>HAALRQPQVAELLAEARRAFREEFGAEPELAVSAPGRVNLIGEHTDYNQGLVLPMALELMTVLVGSPRKDGLVSLLTTSEGADEPQRLQFPLPTAQRSLEPGTPRWANYVKGVIQYYPAAPLPGFSAVVVSSVPLGGGLSSSASLEVATYTFLQQLCPDSGTIAARAQVCQQAEHSFAGMPCGIMDQFISLMGQKGHALLIDCRSLETSLVPLSDPKLAVLITNSNVRHSLASSEYPVRRRQCEEVARALGAASLREVQLE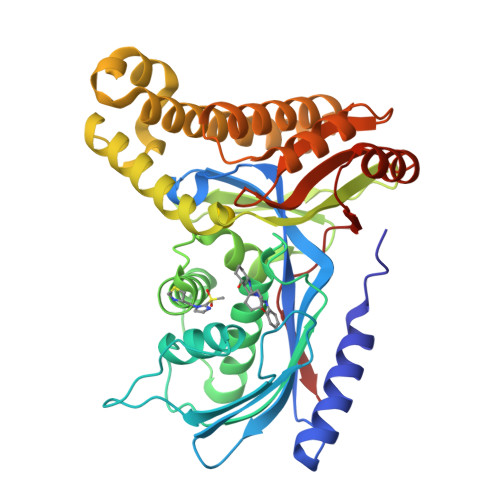ELEAARDLVSKEGFRRARHVVGEIRRTAQAAAALRRGDYRAFGRLMVESHRSLRDDYEVSCPELDQLVEAALAVPGVYGSRMTGGGFGGCTVTLLEASAAPHAMRHIQEHYGGTATFYLSQAADGAKVLCL[4x]> MSVLVYSFASFVLGWCLRSGITYFTRLME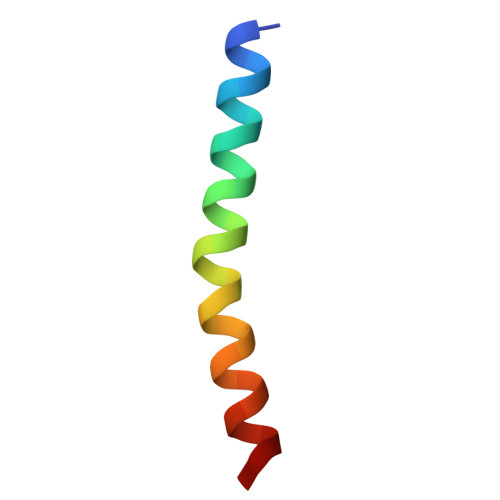TSS>[2x]MTQTFIPGKDAALEDSIARFQQKLSDLGFQIEEASWLNPVPNVWSVHIRDKECALCFTNGKGATKKAALASALGEYFERLSTNYFFADFWLGETIANGPFVHYPNEKWFPLTENDDVPEGLLDDRLRAFYDPENELTGSMLIDLQSGNEDRGICGLPFTRQSDNQTVYIPMNIIGNLYVSNGMSAGNTRNEARVQGLSEVFERYVKNRIIAESISLPE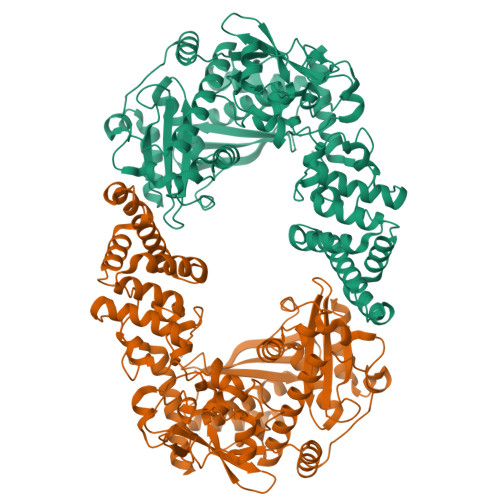IPADVLARYPAVVEAIETLEAEGFPIFAYDGSLGGQYPVICVVLFNPANGTCFASFGAHPDFGVALERTVTELLQGRGLKDLDVFTPPTFDDEEVAEHTNLETHFIDSSGLISWDLFKQDADYPFVDWNFSGTTEEEFATLMAIFNKEDKEVYIADYEHLGVYACRIIVPGMSDIYPAEDLWLANNSMGSHLRETILSLPGSEWEKEDYLNLIEQLDEEGFDDFTRVRELLGLATGSDNGWYTLRIGELKAMLALAGGDLEQALVWTEWTMEFNSSVFSPERANYYRCLQTLLLLAQEEDRQPLQYLNAFVRMYGADAVEAASAAMSGEAAFYGLQPVDSDLHAFAAHQSLLKAYEKLQRAKAAFWAK>AMKLMEVSPLFPCIFLRRVNRFVGLVRIKERIERALITNTGRLNEFMIPGRIGYCTPKAGGKTRYILLGFEDHGKIAIIDTRLQGKAFEKIIEKELLPELEGCRIIKREPRVGESRLDYLIECSKGEIFVETKSAVLREGEYAMYPDCPSVRGQRHIKELIKLARDGKRAMIVFIGALPNVSKFKPYKKGDPKIAELLKEAL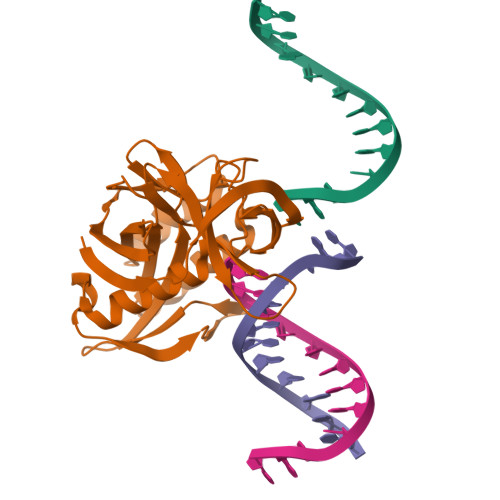EAGVEIRALGLHMELSGEIIYRGELGVEI[2x]> MPEGPEVALTADILEKYFKGKTLEYIDFISGRYSKSEPEGYDDFIANLPLKVSNVDTKGKFLWFELFDPNDKSNKWYIWNTFGLTGMWSLFEAKYTRAVLSFDNELMAYFSDMRNFGTFKFSNSEKELKRKLNELGPDFLKNDDIDISKIKKYKQPIVALLMD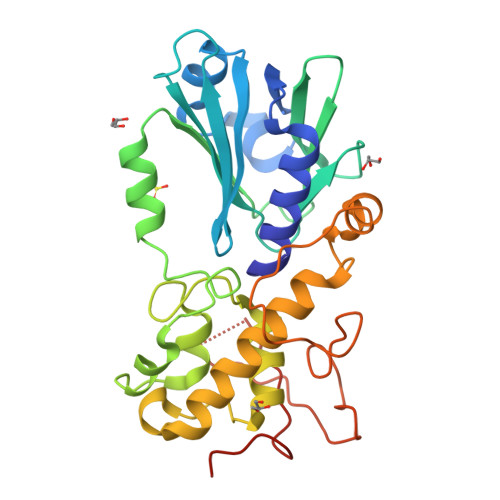QKKIGSGLGNYLVAEILYRAKIDPHKLGSNLTDQEIENLWYWIKYETKLAYDSNHIGYMVNLENESSKIGRKNYHPNIHPTEKEFDFLVYRKKKDPNGNKVIADKIIGSGKNKRTTYWAPAIQKLEHHHHHH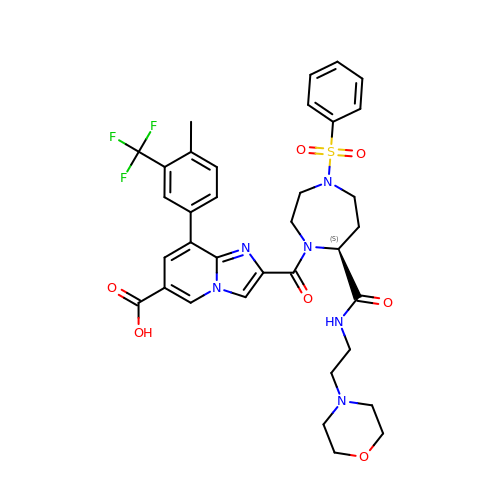8-[4-methyl-3-(trifluoromethyl)phenyl]-2-[[(7S)-7-(2-morpholin-4-ylethylcarbamoyl)-4-(phenylsulfonyl)-1,4-diazepan-1-yl]carbonyl]imidazo[1,2-a]pyridine-6-carboxylic acid | C35 H37 F3 N6 O7 S | CYRHEZSFDUZNDQ-PMERELPUSA-N>QDDASDRQTREVLDPIVASLMEAQQIPGMAIALVRPEGTTISHYGAADRETGTPVDDDTLFEIGSLSKTLTATLASLAEVEGKLDFDAPVSRYLPELEGSAFDDISGLNLGTHTGGGLPLFVPDEVTDRASLMAWYREWQPTEPIGESRTYSNLGIGLLGLETAASLDGEFVPTMRAKVLAPLGMQDTWYDVPEARMADYAMGEDKDGQPTRVSPGVLDDEAYGIKTTAADLAKLVRANLHLADVDAELQQAIDATRQGHYRVGDMTQALIWEQYSLPVAPETLRAGQGYDMILEPNAAEALEPPQSPRDDVWVNKTGSTQGFGGYIVMLPGKHTGLVMLANKNYPNDARVEAAYRILSG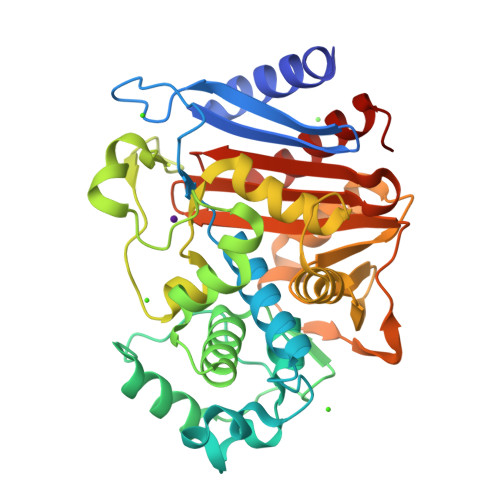LGAIDVP[3x]BAY 1217389 | C27 H24 F5 N5 O3 | 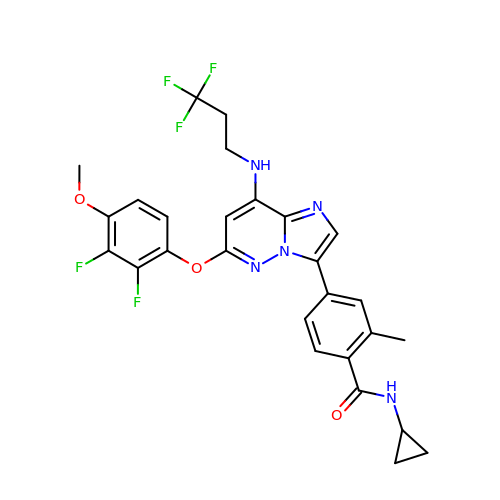WNEILUNVMHVMPH-UHFFFAOYSA-N> NPVENYIDEVLNEVLVVPNIKESHHTTSNSAPLLDAAETGHTSNVQPEDAIETRYVITSQTRDEMSIESFLGRSGCVHISRIKVDYTDYNGQDINFTKWKITLQEMAQIRRKFE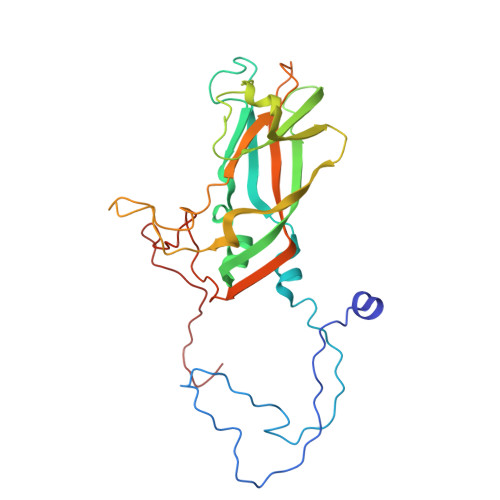LFTYVRFDSEITLVPCIAGRGDDIGHIVMQYMYVPPGAPIPSKRNDFSWQSGTNMSIFWQHGQPFPRFSIPFLSIASAYYMFYDGYDGDNTSSKYGSVVTNDMGTICSRIVTEKQKLSVVITTHIYHKAKHTKAWCPRPPRAVPYTHSHVTNYMPETGDVTTAIVRRNTITTA>[4x]GSNNSETPAPGPDSLLALAFPSDPQVSPDGKQVAFVLAQISEEDPAKPDKDFARPRYRSGLWLSEGGAARPLTHAETGRGDSAPRWSPDGQNLAFVRSAGEVKAALMLLPLKGGEARRVTHFKNGVSGPQWSPDGRFIAF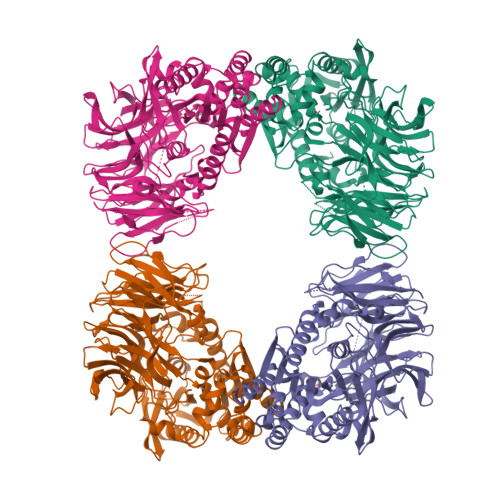TTTADTEDKRDERGEARVLTRPVYRANGADWLPERPAALWLYDVEADKLREWYAPEIGIGALSWWPDSRGVLIVQSEDEWQASQWRQDVYDLPLPTADAPAAPQKLLDWNSAAHGLAPHPDGQRFALIGRPAGKGNTEHAHLYLIENGQHRRLDTGHDHPVGDAVGGDCHVGAFPEGPRWLDGDTLLFSSTVRGSVGLFTAHIGGGVKAYDHDPQGVISAFTANEHGVALIRESATRFPEVELNGQRVTDLHARFPFPVREPQRVTFETELGEGEGWVLLPEGEQKVPALLNIHGGPHTDYGHGFTHEFQLMAARGYGVCYSNPRGSVGYGQAWVDAIYGRWGTVDADDLLNFFDRCLEAVPRLDAAKTAVMGGSYGGFMTNWITGHTTRFQAAITDRCISNLISFGGTSDIGLRFWDDELGLDFSRRADALKLWDLSPLQYVENVKTPTLIVHSVLDHRCPVEQAEQWYAALHKHQVPVRFVRFPEENHELSRSGRPDRRLTRLNEYFAWLERWL allyl (2-(methylamino)-8-oxo-7,8-dihydro-1H-imidazo[4,5-g]quinazolin-6-yl)carbamate | C14 H14 N6 O3 | 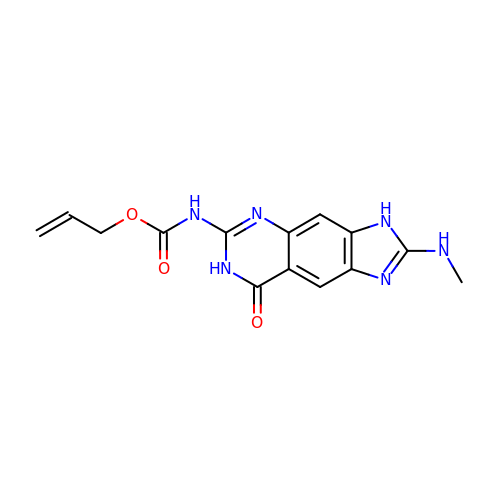SKMZNGUSNLOOPQ-UHFFFAOYSA-N(2E,5R)-2-imino-3-methyl-5-phenyl-5-[3-(pyridin-3-yl)phenyl]imidazolidin-4-one | C21 H18 N4 O 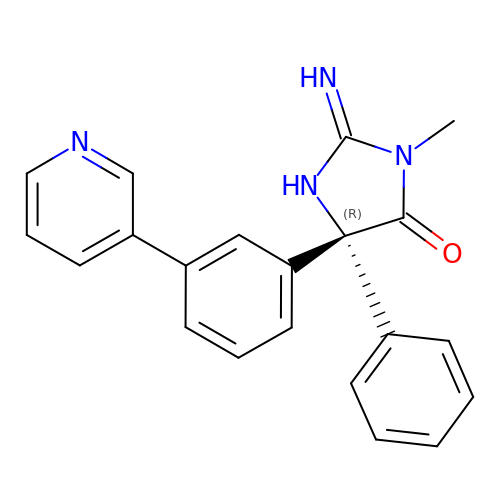| PNSQCPQDRVOKMA-OAQYLSRUSA-N3-(2-chloro-10H-phenothiazin-10-yl)-N,N-dimethylpropan-1-amine 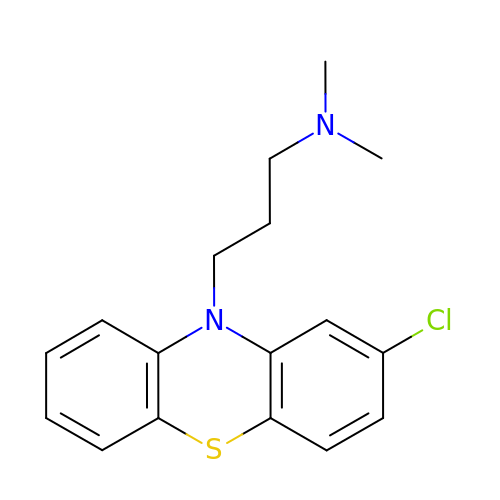| C17 H19 Cl N2 S | ZPEIMTDSQAKGNT-UHFFFAOYSA-N> MKQYLELMQKVLDEGTQKNDRTGTGTLSIFGHQMRFNLQDGFPLVTTKRCHLRSIIHELLWFLQGDTNIAYLHENNVTIWDEWADENGDLGPVYGKQWRAWPTPDGRHIDQITTVLNQLKNDPDSRRIIVSAWNVGELDKMALAPCHAFFQFYVADGKLSCQLYQRSCNVFL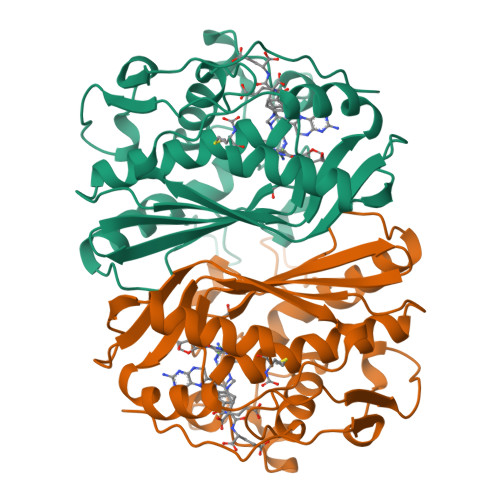GLPFNIASYALLVHMMAQQCDLEVGDFVWTGGDTHLYSNHMDQTHLQLSREPRPLPKLIIKRKPESIFDYRFEDFEIEGYDPHPGIKAPVAI(3R)-3-(fluoromethyl)-3-hydroxy-5-{[(S)-hydroxy(phosphonooxy)phosphoryl]oxy}pentanoic 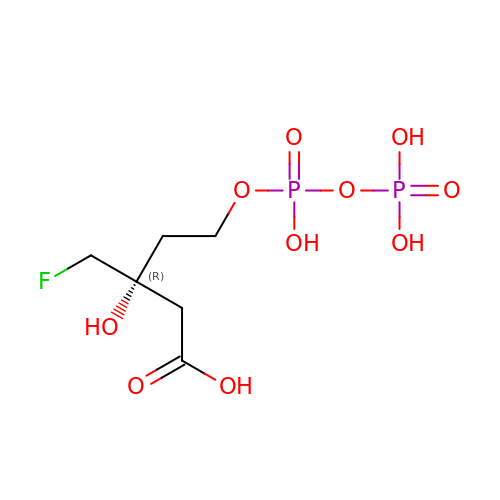acid | C6 H13 F O10 P2 | YIGLDWRZXXHIGZ-ZCFIWIBFSA-N>[4x]MAETEIHTFDDIPMPKLADPLLIY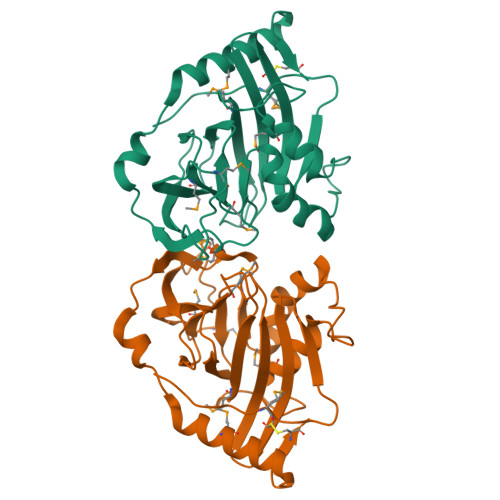TPANEIFDIASCSAKDIGFAIAHAQIPPGGGPMPHIHYFINEWFWTPEGGIELFHSTKQYPNMDELPVVGGAGRGDLYSIQSEPKQLIYSPNHYMHGFVNPTDKTLPIVFVWMRNEVAPDFPYHDGGMREYFQAVGPRITDLNNLPELTNAQRAAFASEAPKYGINQSSYFMEYVNTISDKLPAQIAKLKNDKDLERMVEVIEAFNRGDKSVTCS>MH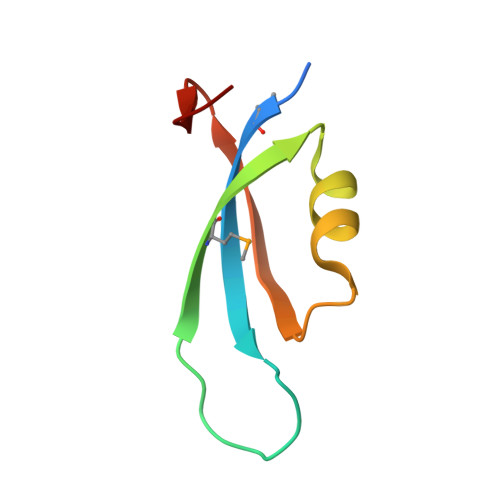HHHHHMIFKVFYQEDADEAPVREKTKTMYIEAESERDVRRKLEGRPINIEYIQPLEGAHLEYE[8x]>[2x]MNTVRSEKDSMGAIDVPADKLWGAQTQRSLEHFRISTEKMPTSLIHALALTKRAAAKVNEDLGLLSEEKASAIRQAADEVLAGQHDDEFPLAIWQTGSGTQSNMNMNEVLANRASELLGGVRGMERKVHPNDDVNKSQSSNDVFPTAMHVAALLALRKQLIPQLKTLTQTLNE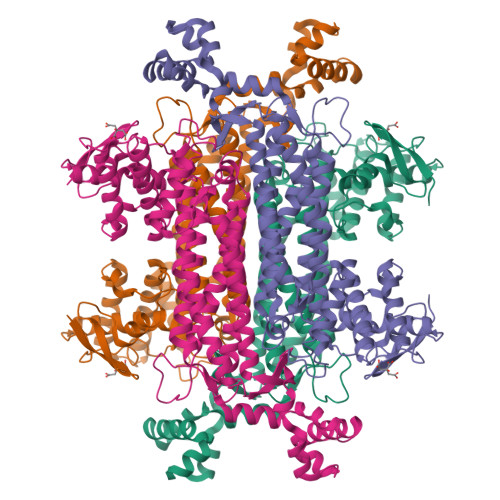KSRAFADIVKIGRAHLQDATPLTLGQEISGWVAMLEHNLKHIEYSLPHVAELALGGTAVGTGLNTHPEYARRVADELAVITCAPFVTAPNKFEALATCDALVQAHGALKGLAASLMKIANDVRWLASGPRCGIGEISIPENEPGSSIMPGKVNPTQCEALTMLCCQVMGNDVAINMGGASGNFELNVFRPMVIHNFLQSVRLLADGMESFNKHCAVGIEPNRERINQLLNESLMLVTALNTHIGYDKAAEIAKKAHKEGLTLKAAALALGYLSEAEFDSWVRPEQMVGSMKAGRPHHHHH>[4x]SVKGS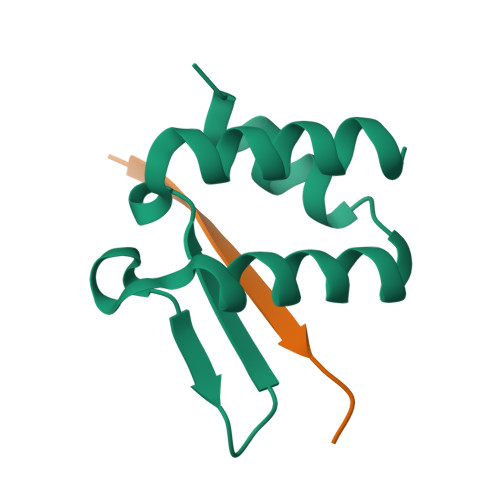VDLEKLAFGLTKLNEDDLVGVVQMVTDNKTPEMNVTNNVEEGEFIIDLYSLPEGLLKSLWDYVKKNT;>EPKLLLKINLKK[4x]>MPSEDYAI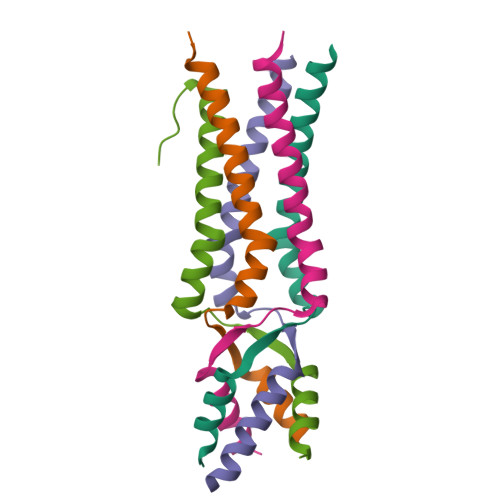WYARATIAALQAAEYRLAMPSASYTAWFTDAVSDKLDKISESLNTLVECVIDKRLAVS[5x]>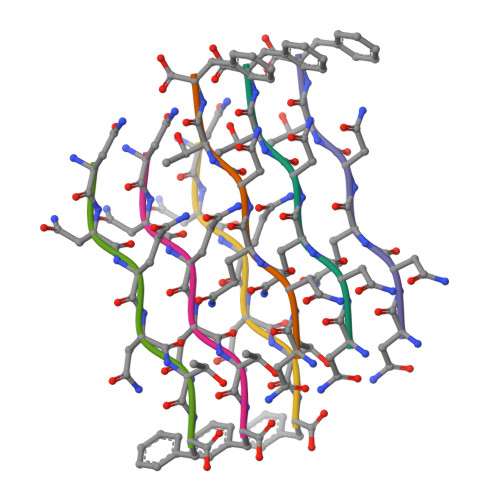 NNQNTF>MGSDKIHHHHHHENLYFQGMNLVQDKVTIITGGTRGIGFAAAKIFID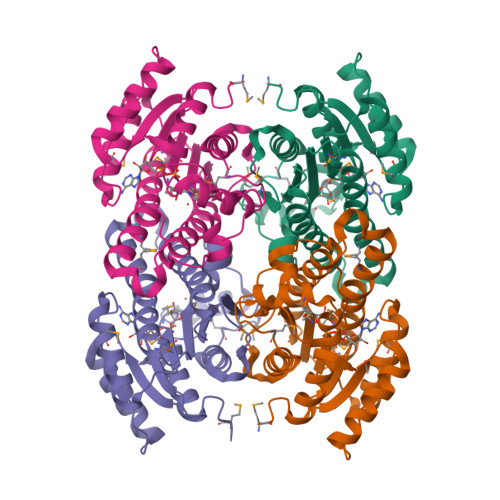NGAKVSIFGETQEEVDTALAQLKELYPEEEVLGFAPDLTSRDAVMAAVGQVAQKYGRLDVMINNAGITSNNVFSRVSEEEFKHIMDINVTGVFNGAWCAYQCMKDAKKGVIINTASVTGIFGSLSGVGYPASKASVIGLTHGLGREIIRKNIRVVGVAPGVVNTDMTNGNPPEIMEGYLKALPMKRMLEPEEIANVYLFLASDLASGITATTVSVDGAYRP[4x]> MADGPSPIRIVLWNDGGESLAAGVEDEEQQQVLHSFADLVGSAIDAVLELPQFRHVEAVTAEAEEDEPGLSIGFDAGSGDGEVDIDNLKGRLDIAGLLLGSAQLPEELAEVAAVEVTDEEEGTTELQFTDEGLVQQLQAVVKRAKLEKRYNDWVAGVAESLGPALDAAAGGVEVTEMPVDPYDVLQAVVAQLIRVAGVSPPAPSLF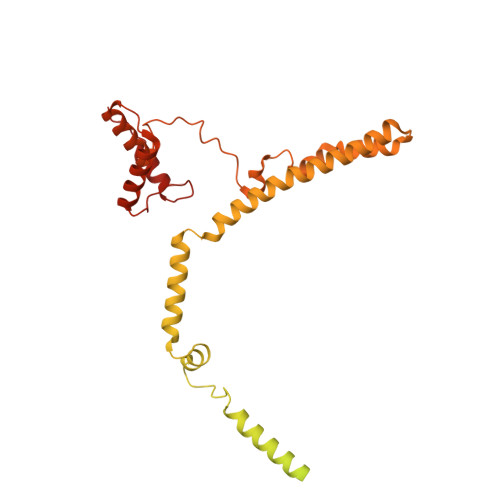SRTGALVGGVLGAPRSAVRQVTKRLGRAQRLWWRLEDVVVDGSKLALRLAVKAARPVLVGFVLHRVLKTLDRSRQLEYRLARMGPEEAREAYYEAVLGKDWKQQLQADWDKALEDVDAGLVTDEINHEKRLMTAAQLRRLEVEEWDKQRMKNFYLASFGGLRWFDQMEQALHNPLFIESRGWTDPVQNWVGQNRTYMDDLPAGQYMAGVGNAAIRIKEAELKRKLTDVERAHVLARGGAVAGGLLPQQPTDPATLAVAVGGAFVPSVAGKR>[2x]MIEIKDKQLTGLRFIDLFAGLGGFRLALESCGAECVYSNEWDKYA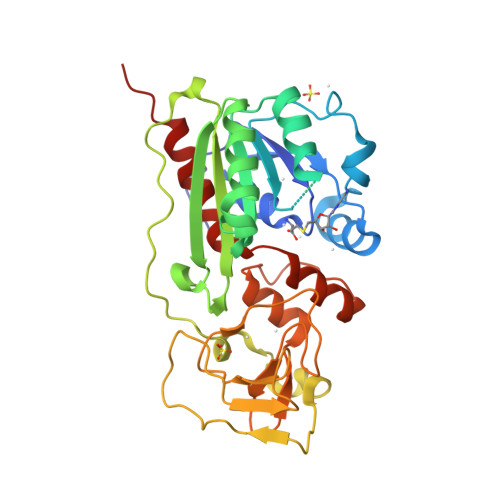QEVYEMNFGEKPEGDITQVNEKTIPDHDILCAGFPCQAFSISGKQKGFEDSRGTLFFDIARIVREKKPKVVFMENVKNFASHDNGNTLEVVKNTMNELDYSFHAKVLNALDYGIPQKRERIYMICFRNDLNIQNFQFPKPFELNTFVKDLLLPDSEVEHLVIDRKDLVMTNQEIEQTTPKTVRLGIVGKGGWGERIYSTRGIAITLSAYGGGIFAKTGGYLVNGKTRKLHPRECARVMGYPDSYKVHPSTSQAYKQFGNSVVINVLQYIAYNIGSSLNFKPY>[2x]MRSKRFEALAKRPVNQDGFVKEWIEEGFIAMESPNDPKPSIKIVNGAVTELDGKPVSDFDLIDHFIARYGINLNRAEEVMAMDSVKLANMLCDPNVKRSEIVPLTTAMTPAKIVEVVSHMNVVEMMMAMQKMRARRTPSQQAHVTNVKDNPVQIAADAAEGAWRGFDEQETTVAVARYAPFNAIALLVGSQVGRPGVLTQCSLEEATELKLGMLGHTCYAETISVYGTEPVFTDGDDTPWSKGFLASSYASRGLKMRFTSGSGSEVQMGYAEGKSMLYLEARCIYITKAAGVQGLQNGSVSCIGVPSAVPSGIRAVLAENLICSSLDLECASSNDQTFTHSDMRRTARLLMQFLPGTDFISSGYSAVPNYDNMFAGSNEDAEDFDDYNVIQRDLKVDGGLRPVREEDVIAIRNKAARALQAVFAGMGLPPITDEEVEAATYAHGSKDMPERNIVEDI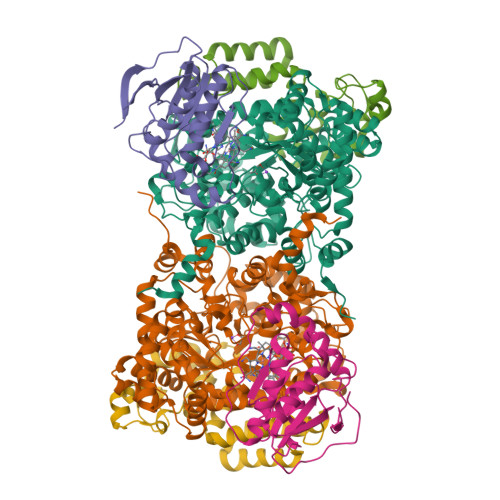KFAQEIINKNRNGLEVVKALAQGGFTDVAQDMLNIQKAKLTGDYLHTSAIIVGDGQVLSAVNDVNDYAGPATGYRLQGERWEEIKNIPGALDPNEID;>[2x]MEINEKLLRQIIEDVLSEMKGSDKPVSFNAPAASAAPQATPPAGDGFLTEVGEARQGTQQDEVIIAVGPAFGLAQTVNIVGIPHKSILREVIAGIEEEGIKARVIRCFKSSDVAFVAVEGNRLSGSGISIGIQSKGTTVIHQQGLPPLSNLELFPQAPLLTLETYRQIGKNAARYAKRESPQPVPTLNDQMARPKYQAKSAILHIKETKYVVTGKNPQELRVAL;>MNTDAIESMVRDVLSRMNSLQGEAPAAAPAAGGASRSARVSDYPLANKHPEWVKTATNKTLDDFTLENVLSNKVTAQDMRITPETLRLQASIAKDAGRDRLAMNFERAAELTAVPDDRILEIYNALRPYRSTKEELLAIADDLESRYQAKICAAFVREAATLYVERKKLKGDD[2x]> MADLAECNIKVMCRFRPLNESEVNRGDKYIAKFQGEDTVVIASKPYAFDRVFQSSTSQEQVYNDCAKKIVKDVLEGYNGTIFAYGQTSSGKTHTMEGKLHDPEGMGIIPRIVQDIFNYIYSMDENLEFHIKVSYFEIYLDKIRDLLDVSKTNLSVHEDKNRVPYVKGCTERFVCSPDEVMDTIDEGKSNRHVAV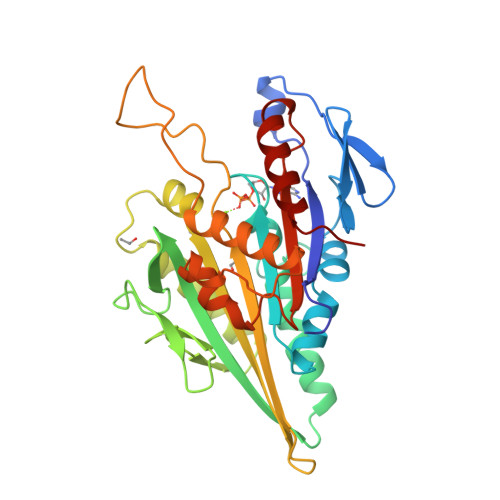TNMNEHSSRSHSIFLINVKQENTQTEQKLSGKLYLVDLAGSEKVSKTGAEGAVLDEAKNINKSLSALGNVISALAEGSTYVPYRDSKMTRILQDSLGGNCRTTIVICCSPSSYNESETKSTLLFGQRAKTI> NSPHSRAMYVYPPNVESSPELPKHIYNKLDKGQIIVVIWV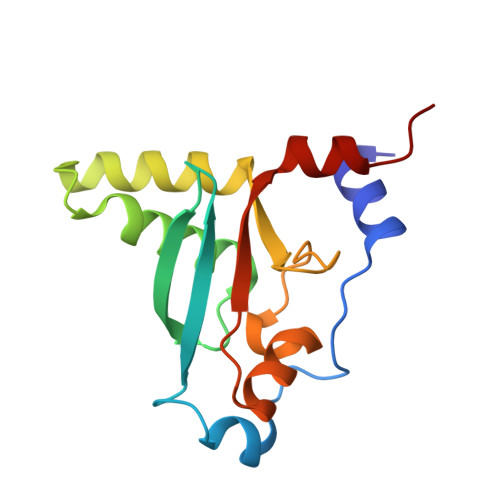IVSPNNDKQKYTLKINHDCVPEQVIAEAIRKKTRSMLLSSEQLKLCVLEYQGKYILKVCGCDEYFLEKYPLSQYKYIRSCIMLGRMPNLMLMAKESLYSQLPMD>MATPVTIYGPPLCTAVSRVLATLIEKDVPFHLIPIDLSKGEQKKPEYLKIQPFGQVPAFKDESITLFESRAICRYICDKYADKGNKSLYGTDILSKANIDQWVETDGQTFGPPSGDLVHDLLFSSVPVDEALIKKNVDKLAKVLDIYEQKLGQTRFLAGDEFSFADLSHLPNGDYLVNSTDKGYLFTSRKNVNRWWTEISNRESWKKVLEMRKNA[2x]

Glutathione transferases (GSTs; EC 2.5.1.18) represent a ubiquitous multigenic family of enzymes that conjugate the reduced tripeptide glutathione (GSH, γ-Glu-Cys-Gly) on a wide range of endogenous and exogenous electrophilic molecules. At the structural level, GSTFs exist as homodimers, the dimerization interface involving mainly hydrophobic surface patches. Each monomer comprises an active site region formed by a glutathione binding pocket (G-site) primarily involving residues from the conserved N-terminal thioredoxin domain and an hydrophobic pocket (H-site) primarily involving residues from the less conserved C-terminal domain. A PttGSTF1 monomer consists of an N-terminal domain (β1α1β2α2β3β4α3) and a C-terminal domain composed of α-helices (α4α5α6α6′α7α8) as classically observed in most GST classes.

In order to investigate the biochemical and structural properties of GSTF1, the mature form was expressed in E. coli as well as single mutated protein variants, the catalytic serine of which was replaced by a cysteine or an alanine residue. A mass increment of 305 Da was specifically present in PttGSTF1 S13C, which suggested that a glutathione molecule is covalently bound to the newly introduced cysteine residue via a disulfide bridge. Accordingly, PttGSTF1 S13C is not retained on GSH Sepharose columns contrary to PttGSTF1 and PttGSTF1 S13A. Concerning PttGSTF1 S13C, the structure refinement confirmed that Cys13 is glutathionylated but this modification did not induce significant conformational changes in comparison to PttGSTF1 (RMSD of 0.33Å based on alignments of 350 Cα positions). According to mass spectrometry data, in the PttGSTF1 S13C variant, GSH is covalently bound to the modified residue (Cys13). Apart this difference, the same GSH-protein interactions are observed in both crystal structures. Whereas this suggested that one or several residues other than the serine contribute to the decrease of the pKa of the thiol group of GSH, the PttGSTF1 S13C variant had no or negligible activity toward all these substrates. Concerning PttGSTF1 S13C, whereas no activity has been detected with DHA, a reasonably good catalytic efficiency (1.1 × 103 M−1 s−1) was obtained with HED, essentially because of a good apparent affinity (Km value of 33.7 μM). Another proof of this assumption is that the PttGSTF1 S13C mutant lost its glutathione peroxidase and glutathionylating activity but acquired the capacity to perform deglutathionylation reaction toward HED, an activity typical of Cys-GSTs. Although the detected activity is weaker than the one obtained with naturally-existing Cys-GSTs, it shows that changing the nature of the catalytic residue is sufficient to determine the type of GST activity.> DYKDDDDLHSQANLMRLKSDLFNRSPMYPGPTKDDPLTVTLGFTLQDIVKADSSTNEVDLVYYEQQRWKLNSLMWDPNEYGNITDFRTSAADIWTPDITAYSSTRPVQVLSPQI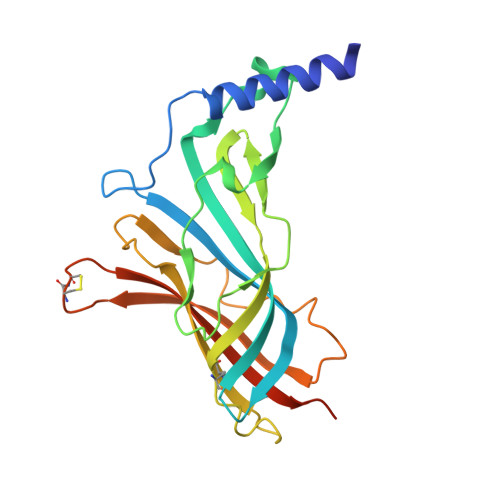AVVTHDGSVMFIPAQRLSFMCDPTGVDSEEGATCAVKFGSWVYSGFEIDLKTDTDQVDLSSYYASSKYEILSATQTRQVQHYSCCPEPYIDVNLVVKFRERRAGNGFFRNLFD>SMGFWEASSRGGGAFSGGEDASEGGAEEGAGGAGGSAGAGEGPVITALTPMTIPDVFPHLPLIAITRNPVFPRFIKIIEVKNKKLVELLRRKVRLAQPYVGVFLKRDDSNESDVVESLDEIYHTGTFAQIHEMQDLGDKLRMIVMGHRRVHISRQLEVEPEEPEAENKHKPRRKSKRGKKEAEDELSARHPAELAMEPTPELPAEVLMVEVENVVHEDFQVTEEVKALTAEIVKTIRDIIALNPLYRESVLQMMQAGQRVVDNPIYLSDMGAALTGAESHELQDVLEETNIPKRLYKALSLLKKEFELSKLQQRLGREVEEKIKQTHRKYLLQEQLKIIKKELGLEKDDKDAIEEKFRERLKELVVPKHVMDVVDEELSKLGLLDNHSSEFNVTRNYLDWLTSIPWGKYSNENLDLARAQAVLEEDHYGMEDVKKRILEFIAVSQLRGSTQGKILCFYGPPGVGKTSIARSIARALNREYFRFSVGGMTDVAEIKGHRRTYVGAMPGKIIQCLKKTKTENPLILIDEVDKIGRGYQGDPSSALLELLDPEQNANFLDHYLDVPVDLSKVLFICTANVTDTIPEPLRDRMEMINVSGYVAQEKLAIAERYLVPQARALCGLDESKAKLSSDVLTLLIKQYCRESGVRNLQKQVEKVLRKSAYKIVSGEAESVEVTPENLQDFVGKPVFTVERMYDVTPPGVVMGLAWTAMGGSTLFVETSLRRPQDKDAKGDKDGSLEVTGQLGEVMKESARIAYTFARAFLMQHAPANDYLVTSHIHLHVPEGATPKDGPSAGCTIVTALLSLAMGRPVRQNLAMTGEVSLTGKILPVGGIKEATIAAKRAGVTCIVLPAENKKDFYDLAAFITEGLEVHFVEHYREIFDIAFPDEQAEALAVER[6x]

The hexameric, barrel-forming, AAA+ protease Lon is critical for maintaining mitochondrial matrix protein homeostasis. A human Lon monomer contains a mitochondrial targeting sequence, a Lon-associated N-terminal (LAN) domain, an α-helical neck region, an AAA+ domain, and a protease domain (PD) in a single chain. The LAN domains specifically recognize and capture fully or partially unfolded substrates, which are then threaded towards the barrel chamber for degradation using the chemical energy from ATP hydrolysis. We determined high-resolution structures of substrate-engaged, substrate-trapped, and substrate-free forms of the human mitochondrial Lon protease.

Nucleophilic attack of S855 on the peptide bond creates an ester linkage between Lon and the substrate. The enzyme-substrate intermediate is resolved with the help of K898, which activates a water molecule for nucleophilic attack on the ester. Therefore, we introduced the mutation K898A (Lon^K898A^) in wt-Lon to trap the enzyme-substrate covalent intermediate of the hydrolysis reaction. We determined the structure of Lon^K898A^ in a similar manner to Lon^SE^ and the reconstruction revealed clear density for a trapped substrate in the protease domain. The trapped substrate is present in all six protomers, but its signal is approximately five-fold lower than that of the surrounding PD atoms. This suggests that only one of the six catalytic sites is occupied in each Lon particle. We modelled tetra-alanine peptides in the maps and they show a β-strand conformation with the C-terminus of the substrate reaching S855 ([Fig fig4]) and the N-terminus pointing towards the centre of the barrel. In contrast, the gate loop adopts an open conformation in Lon^SE^ and Lon^K898A^, in which the catalytic site is exposed ([Fig fig4]). Furthermore, reconstruction of covalently-trapped Lon^K898A^ obtained in the presence of substrate TFAM retains the in-plane six-fold symmetry of the PDs and shows substrate density in all protease domains. After the covalent bond between S855 and the TFAM C-terminus forms, substrate threading is stalled.> AGCCAGCCTGTACGGACATCA;> CC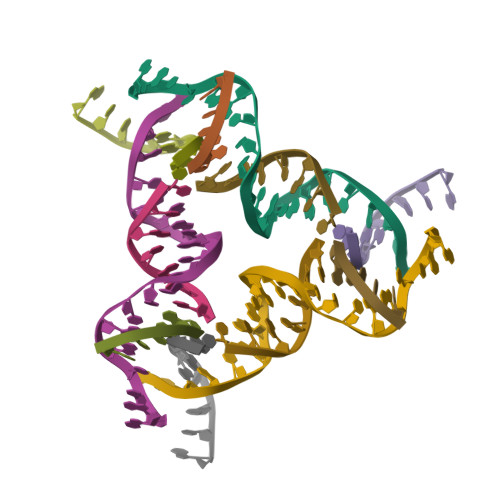GTACA;> GGCTG;> GTCTGATGT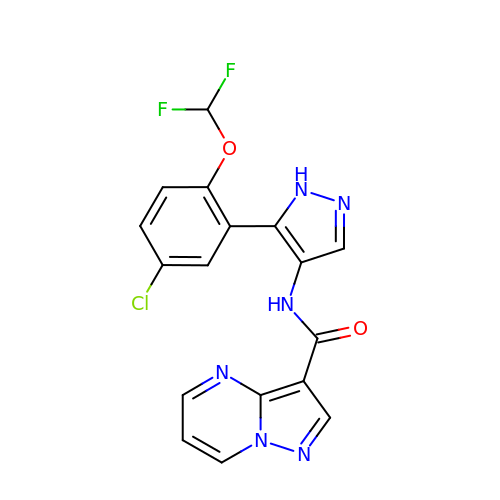N-{5-[5-chloro-2-(difluoromethoxy)phenyl]-1H-pyrazol-4-yl}pyrazolo[1,5-a]pyrimidine-3-carboxamide | C17 H11 Cl F2 N6 O2 | KHCFKCPXXJQHMH-UHFFFAOYSA-N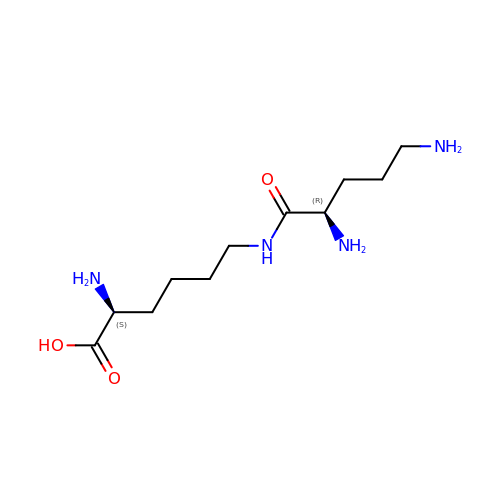N~6~-D-ornithyl-L-lysine | C11 H24 N4 O3 | AOOVWOOUTNDWMA-BDAKNGLRSA-N>MSSFVPNKEQTRTVLIFCFHLKKTAAESHRMLVEAFGEQVPTVKTCERWFQRFKSGDFDVDDKEHGKPPKRYEDAELQALLDEDDAQTQKQLAEQLEVSQQAVSNRLREMGKIQKVGRWVPHELNERQMERRKNTCEILLSRYKRKSFLHRIVTGDEKWIFFVNPKRKKSYVDPGQPATSTARPNRFGKKTMLCVWWDQSGVIYYELLKPGETVNAARYQQQLINLNRALQRKRPEYQKRQHRVIFLHDNAPSHTARAVRDTLETLNWEVLPHAAYSPDLAPSDYHLFASMGHALAEQRFDSYESVKKWLDEWFAAKDDEFYWRGIHKLPERWEKCVASDGKYFE[2x]

Mariner/Tc1/IS630 family transposases are unusual as they integrate their transposons, with a 2 bp stagger, strictly at TA target sequences. The wealth of structural and biochemical data for the naturally active, eukaryotic transposon Mos1 offers a paradigm for determining the molecular mechanism of mariner/Tc1 transposon integration. The 1286 bp transposon is framed by 28 bp imperfect inverted repeats (IR) and encodes a 345 amino acid transposase that can perform cut-and-paste DNA transposition in vitro, as shown in Figure 1a. The Mos1 transposase homodimer binds to the IR at one transposon end and then captures the other IR, forming a paired-end complex (PEC). After excision, the Mos1 transpososome locates a TA target integration site and, upon binding, forms a target capture complex (TCC).

To assemble the Mos1 STC, full length T216A Mos1 transposase was combined, in a 1:1 molar ratio, with DNA representing the product of transposon integration. This DNA contains the transposon IR joined at its 3' end to an unpaired TA dinucleotide and target DNA. The refined Mos1 STC crystal structure contains a transposase homodimer bound to two DNA duplexes representing the products of transposon integration. Target DNA binds in a channel between the two catalytic domains and the active sites contain the strand transfer products. The transposase subunits adopt a crossed (or trans) arrangement with IR DNA in the Mos1 STC, similar to the pre- and post-TS cleavage Mos1 PECs: each IR is recognised by the DNA-binding domain of one transposase subunit and by the catalytic domain of the other subunit, and vice versa. The target DNA is severely distorted from B-form conformation: the backbone is bent by 147°, with the apex of the bend at the TA target dinucleotide. The most striking feature of the Mos1 STC structure is flipping of both target adenine (A1) bases of the symmetrical TA sequence into extra-helical positions. The aromatic ring of each F187 occupies the space vacated by a flipped A1, forming a π–π stack with the adjacent G2 nucleobase, stabilising this conformation. Side-chain atoms of transposase residues R186, K190 and W159 stabilise these distortions by forming salt bridges or hydrogen bonds with the A1 and G2 phosphates. One Mg2+ was observed in each active site in the Mos1 STC, coordinated by the D156 and D249 carboxylates, the 3'-OH of C-1 and a water molecule.> TQKSLSKEEIERYSRQMIVPGMGKEGQLRLMNAKVLIIGAGGLGCPAAQYLAGAGVGTIGIVDGDSVETSNLHRQVAHATKRVGMLKVDSLITHLIEINPLPVYVPYRFDLTPQNAAQIIKPWDVILDCTDNPATRYLISDVCVLLGKPLVSAASVQKSGQLIVLNCPPTPQGVVNKKAAP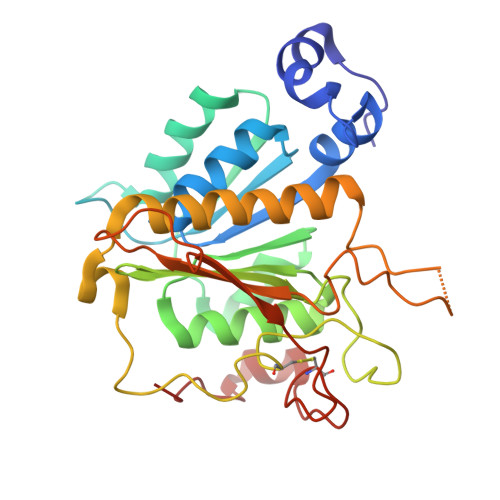CYRCCFKKPPPPSAQTSKGEAGIMGPVVGMMGVAQAGEAIKILVSQLHMPPKEGEEVSPEKNLVQPTLLIYTYDLNSAIGPYSFRALKMGGRKKDCFACGENSTLTLDGIKSGNPNYVQF> NFDYMFKILIIGNSSVGKTSFLFRYADDSFTPAFVSTVGIDFKVKTIYRNDKRIKLQIWDTAGQERYRTITTAYYRGAMGFILMYDITNEESFNAVQDWSTQIKTYSWDNAQVLLVGNKCDME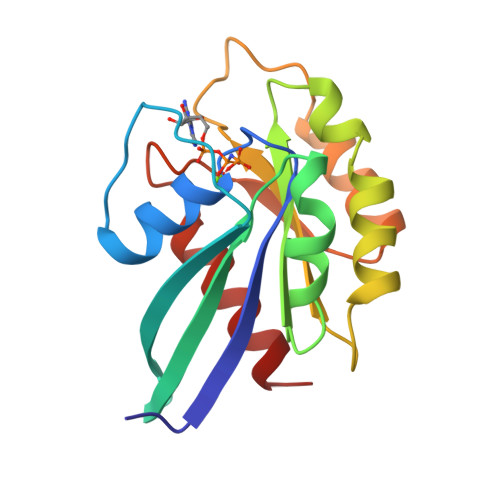DERVVSSERGRQLADHLGFEFFEASAKDNINVKQTFERLVDVICEK> GTQSLNPHNDYCQHFVDTGHRPQNFIRDVGLADRFEEYPKLRELIRLKDELIAKSNTPPMYLQADIEAFDIRELTPKFDVILLEPPLEEYYRETGITANEKCWTWDDIMKLEIDEIAAPRSFIFLWCGSGEGLDLGRVCLRKWGYRRCEDICWIKTNKNNPGKTKTLDPKAVFQRTKEHCLMGIKGTVKRSTDGDFIHANVDIDLIITEEPEIGNIEKPVEIF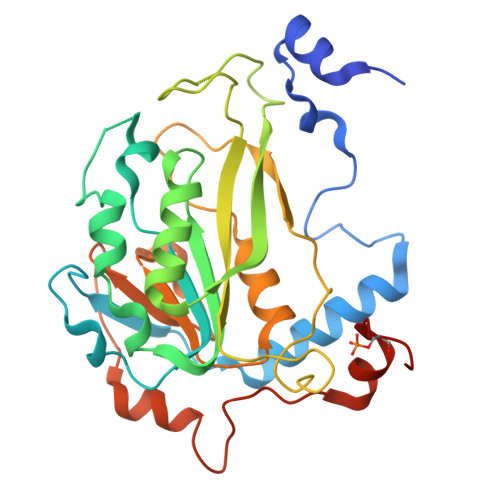HIIEHFCLGRRRLHLFGRDSTIRPGWLTVGPTLTNSNYNAETYASYFSAPNSYLTGCTEEIERLRPKSPPPKSKSDR>[12x]MKSVVTTVIAAADAAGRFPSSSDLESVQGSIQRSAARLEAAEKLAGNIDAVAQEAYNACIQKYPYLNNSGEANSTDTFKAKCLRDVKHYMRLIQYSLVVGGTGPLDEWGIAGQREVYRALGLPTAPYVEALSFARNRGCAPRDMSAQALTEYNALLDYAINSLS;>[12x]MLDAFSRAVVQADASTSVVADMGALKQFIAEGNRRLDAVNAIASNASCMVSDAVAGMICENQGLIQAGGNCYPNRRMAACLRDAEIILRYVTYALLAGDASVLDDRCLNGLKETYAALGVPTTSTVRAVQIMKAQAAAHIKDTPSEARAGGKLRKMGSPVVEDRCASLVAEASSYFDRVISALS

The major light-harvesting complexes of cyanobacteria and red algae are the phycobilisomes. These large, water-soluble pigment–protein complexes bind to the surface of the photosynthetic membranes and funnel absorbed light energy into the chlorophyll-containing photosystems. PEs are oligomers of a basic heterodimer that consists of α- and β-subunits (conventionally referred as αβ monomer) to which bile pigments are covalently attached through conserved cysteine residues. For example, see the quantum mechanics/molecular mechanics calculations performed for the cryptophyte PE545 antenna (Aghtar et al. 2017; Curutchet and Mennucci 2017 and other references within) based on the 0.97 Å resolution structure of PE545 from unicellular cryptophyte Rhodomonas CS24. In the case of PE from Phormidium sp. A09DM the pigment present is phycoerythrobilin (PEB) bound covalently to PE protein via one or two CPEB–SCys bonds; its structure is shown in Fig. 1.

The description of the atomic resolution structure of PE will be presented here using the model based on the 1.14 Å data for the crystal grown in NPS conditions (Morpheus C8) while the model based on the 1.38 Å data (crystal grown in carboxylic acids mix, Morpheus G8) will only be mentioned explicitly in the cases of significant structural differences. However, another of the two PE structures we are reporting here, the one refined based on the 1.38 Å data obtained for the crystal grown in the mix of carboxylic acids (Morpheus screen G8 condition) presents another case. In that structure, the conformation of the 146–152 fragment of the loop in β-subunits M and X is the same as in the 1.14 Å structure, but the situation in β-subunits N to W is different. Another more tentative binding site for phosphate was also identified in the α-subunit forming H-bonds with residues Gly112, Arg114 and Glu115. Both these sites are close to the central cavity inside each trimer.> MRGSHHHHHHGSMAEGEEYDKILVLNFGSQYFHLIVKRLNNIKIFSETKDYGVELKDIKDMNIKGVILSGGPYSVTEAGSPHLKKEVFEYFLEKKIPIFGIAYGMQEIAVQMNGEVKKSKTSEYGATDVNILRNDNINNITYCRNFGDSSSAMDLYSNYKLMNETCCLFENIKSDITTVWMNHNDEVTKIPENFYLVSSSENCLICSIYNKEYNIYGVQYHPEVYESLDGELMFYNFAYNICKCKKQFDPIRYHELELKNIEKYKHDHYVIAAMSGGIDSTVAAAYTHKIFKERFFGIFIDNGLLRKNEAENVYTFLKSTFPDMNITKIDASENFLSNLQGVTDPEQKRKIIGKLFIEEFEKAVNNIDIDINKTFLLQGTLYPDIIESK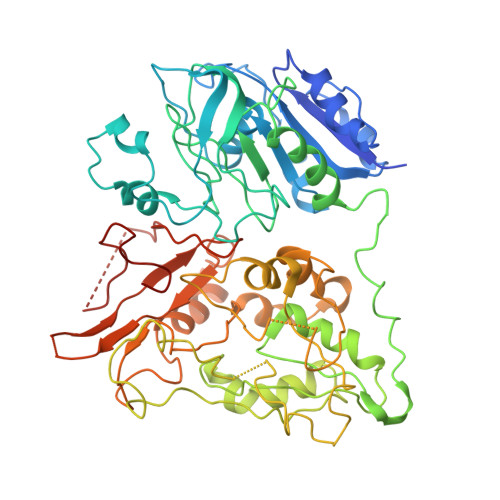CSKNLSDTIKTHHNVGGLPKNLKFKLFEPFKYLFKDDVKTLSRELNLPEEITNRHPFPGPGLAIRVIGEINKHKLNILREVDDIFINDLKQYGLYNQISQAFAVLLSSKSVGVRGDARSYDYVCVLRAVKTSSFMTANWYQIPYDILDKITTRILSEVKGVNRILYDVSSKPPATIEFE> AAGVAAWLPFARAAAIGWMPVASGPMPAPPRQERKRTQDALIVLNVSGTRFQTWQDTLERYPDTLLGSSERDFFYHPETQQYFFDRDPDIFRHILNFYRTGKLHYPRHECISAYDEELAFFGLIPEIIGDCCYEEYKDRRRENAERLQDDADTDTAGESALPTMTARQRVWRAFENPHTSTMALVFYYVTGFFIAVSVIANV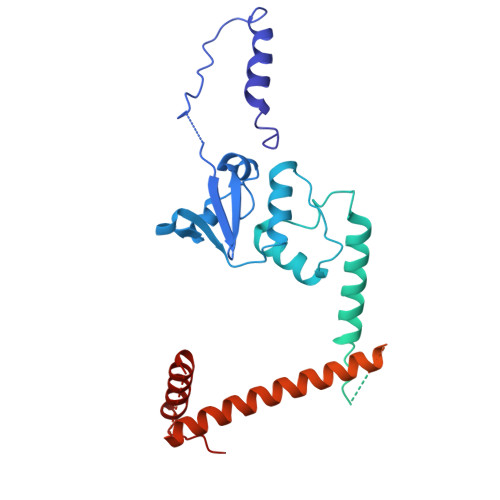VETVPCGSSPGHIKELPCGERYAVAFFCLDTACVMIFTVEYLLRLAAAPSRYRFVRSVMSIIDVVAILPYYIGLVMTDNEDVSGAFVTLRVFRVFRIFKFSRHSQGLRILGYTLKSCASELGFLLFSLTMAIIIFATVMFYAEKGSSASKFTSIPAAFWYTIVTMTTLGYGDMVPKTIAGKIFGSICSLSGVLVIALPVPVIVSNFSRIYHQNQRADKRRAQKKARLARIRAAKSGSANAYMQSKRSGLLSNQLQSSEDEQAFVSKSGSSFETQHHHLLHCLEKTTNHEFVD> PDVVLVNGGEPPNPLIPTGTNDSNGGRIIDRLFAGLMSYDAVGKPSLEVAQ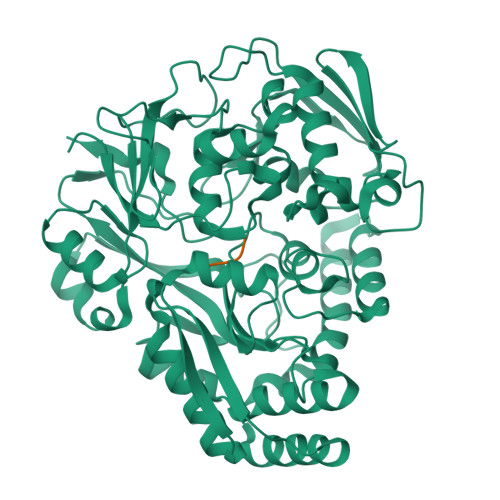SIESADNVNYRITVKPGWKFTDGSPVTAHSFVDAWNYGALSTNAQLQQHFFSPIEGFDDVAGAPGAASRTTMSGLRVVNDLEFTVRLKAPTIDFTLRLGHSSFYPLPDSAFRDMAAFGRNPIGNGPYKLADGPAGPAWEHNVRIDLVPNPDYHGNRKPRNKGLRFEFYANLDTAYADLLSGNLDVLDTIPPSALTVYQRDLGDHATSGPAAINQTLDTPLRLPHFGGEEGRLRRLALSAAINRPQICQQIFAGTRSPARDFTARSLPGFDPNLPGNEVLDYDPQRARRLWAQADAISPWSGRYAIAYNADAGHRDWVDAVANSIKNVLGIDAVAAPQPTFAGFRTQITNRAIDSAFRAGWRGDYPSMIEFLAPLFTAGAGSNDVGYINPEFDAALAAAEAAPTLTESHELVNDAQRILFHDMPVVPLWDYISVVGWSSQVSNVTVTWNGLPDYENIVKA;> SSVT>GSHMVTDRDRLRPPLDERSLRDQLIGAGSGWRQLDVVAQTGSTNADLLARAASGADIDGVVLIAEHQTAGRGRHGRGWAATARAQIILSVGVRVVDVPVQAWGWLSLAAGLAVLDSVAPLIAVPPAETGLKWPNDVLARGGKLAGILAEVAQPFVVLGVGLNVTQAPEEVDPDATSLLDLGVAAPDRNRIASRLLRELEARIIQWRNANPQLAADYRARSLTIGS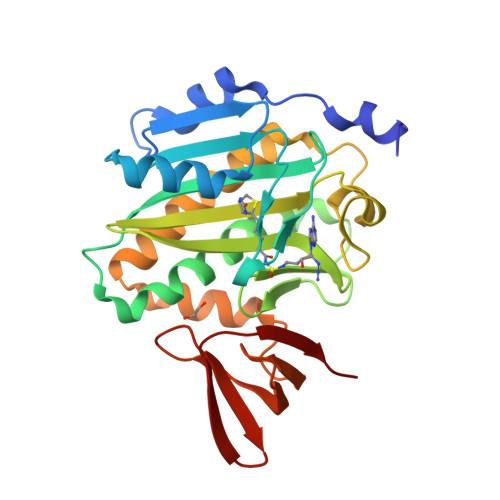RVRVELPGGQDVVGIARDIDDQGRLCLDVGGRTVVVSAGDVVHLR[2x]> MSGGTPEERLAQLEKEIQALYDAADEVVDEVEEKDGKMTVTRTLTIGDGTVTLVETLKIVDGAPVKDGEIEVICNPECEELGKRLKALAKEYEKAQEEVEKAKA;> LKCNQLIPPFWKTCPKG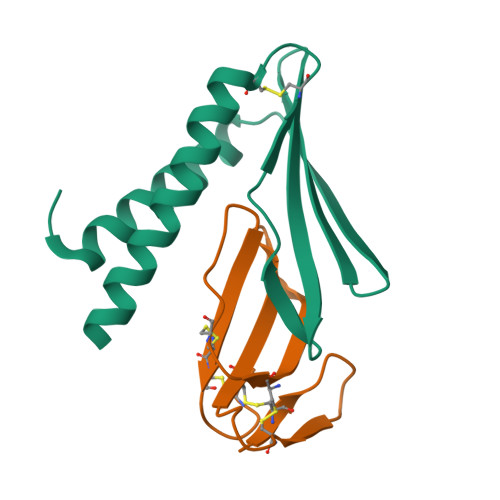KNLCYKMTMRAAPMVPVKRGCIDVCPKSSLLIKYMCCNTDKCN> MIELPVVNPDGAETPGSGKRLWRSTADLRRDPEWVKLAHDEFMPGVAEPPSGTSRRQFLQIMGASMALAGLTACRRPVEKILPYVRQPEEIIPGIPLYYATAMPFRGSVRPLLVESHEGRPTKIEGNPDHPLSRGATGVFEQASLLNLYDPDRSQQVLRKGEPASWGDFVQFARSLAAEAGTKRLAVLCEPSSSPTLAALRRELERRYAQVRWVTYRPEGDDHEALGLQQAFGRPVRARYRFSEARVIVSLDADFLGPTDRNFVENTREFAASRRMERPEDEISRLYVIESTYTVTGGMADHRLRLRAGDIPAFAAALAAELGVGELREAGARFAGHPYVVEIARDLRAAGARGVVLAGETQPPAVHALCAVINDLLGSLGRTVILHAL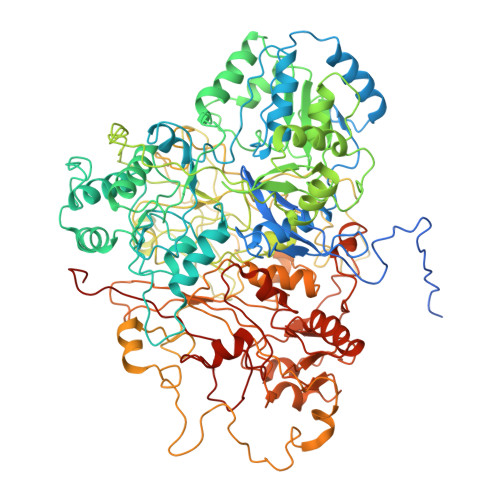DEPATAQHAALAELVQAMQAGAVDALLLLNVNPVYDAPAALGFAEALAQVPEVIHLGLHVDETARRSTWHLPSTHYLEAWGDGRAYDGTLSVIQPLIAPLYEAAHSPLEVLALLATGEEQSAYDLVRNTWRRLLAGRGAFEQAWQRVLHDGFLPDSGYPTVSLRPNRQALADWPQAAEGGLEVVFRLDPTVLDGSFANNAWAQELPDPITKIVWDNVAILSPKTAAALGVKAEYHKGVYIADVIELSLDGRAVELPVWVLPGHPDDSITVYLGYGREITSTRPERKTPFFDLDDYTDIYGHGAIATGVGVNVAPLRRPDNTWVAYGAQVRKTGRTYKIVTTQDHGSMVGRPLVRLATVEEFRKNPDFAKEAEPPLEGLEPWDQYPTLWEENHPSKQPAFQDSDYYRNQWAMVIDLNACTGCNACIVACDSENNIPMVGKNEVGRGREMHWLRIDRYFVSDEAHADDPQIVVQPVPCMHCENAPCESVCPVAATVHSPDGLNEMVYNRCIGTRYCSNNCPYKVRRFNWFNWVKTLPIQVQMAQNPDVTVRFRGVMEKCTYCVQRIREAQRQANIEKRPLRDGEVKTACQQACPAEAITFGDLNDPNNAVVKQRQNARRYEMLAALNVKPRTSYLARITNPNPRLLEQEPVA> GNLPPEKKWLGTPIEEMRKMPRCGIHLPSLRPSASHTVTVRVDLLRAGEVPKPFPTHYKDLWDNKHVKMPCSEQNLYPVEDENGERTAGSRWELIQTALLNKFTRPQNLKDAILKYNVAYSKKWDFTALVDFWDKVLEEAEAQHLYQSILPDMVKIALCLPNICTQPIPLLKQKMNHSVTMSQEQIASLLANAFFCTFPRRNAKMKSEYSSYPDINFNRLFEGRSSRKPEKLKTLFCYFRRVTEKKPTGLVTFTRQSLEDFPEWERCEKPLTRLHVTYEGTIEGNGRGMLQVDFANRFVGGGVTGAGLVQNEIRFLINPELIVSRLFTEVLDHNECLIITGTEQYSEYTGYAETYRWARSHEDGSEKDDWQRRCTEIVAIDALHFRRYLDQFVPEKVRRELNKAYCGFLRPGVPSENLSAVATGNWGCGAFGGDARLKALIQILAAAAAERDVVYFTFGDSELMRDIYSMHTFLTERKLDVGKVYKLLLRYYNEECRNCSTPGPDIKLYPFIYHAVESSAET

Reversal of PARylation is predominantly carried out by poly(ADP-ribose) glycohydrolase (PARG) in nucleus and cytosol, whereas ADP-ribosylhydrolase 3 (ARH3) may play a role in mitochondrial PAR degradation. PARG comprises an N-terminal regulatory/targeting domain and a C-terminal catalytic domain. The mouse PARG catalytic domain has a bean-shaped structure, with the active site in a deep cleft in the middle on the abdominal side.

To understand what caused the activity difference between the mPARG E748N/Q and E749N/Q mutants, we solved the crystal structures of these mPARG mutants. Interestingly, while E748N and E749N mutants were completely dead, both E748Q and E749Q mutants still retained residual PARG activities. In contrast, the signature loops in E748N and E749N mutants have significantly different conformation from the wild type PARG. In wild-type PARG structure, Cβ and Cγ of both E748 and E749 residues are semi-buried. Mutation to Asn, which has both Cγ and Nγ linked to Cβ causes a spatial collision. Therefore, the conformation changes in this catalytic loop completely abolish activity of mPARG E748N and E749N mutants. To study the enzymatic mechanism of mPARG, we tried to soak the catalytic residue Glu748, Glu749 mutants E748N, E748Q, E749N and E749Q with the iso-ADPr, which may be the smallest PARG substrate containing the α(1→2) ribose-ribose glycosidic bond to be cleaved by PARG. In all above four PARG mutant crystal structures, we were not able to observe the electron density for iso-ADPr at the “active” site of mPARG. For E748N and E749N mutants, this may result from the conformational change in the active site associated with the mutation. Our work revealed precisely how some of the PARG mutations (e.g. E748N, E749N) disrupt the PARG activity through significant conformational changes in the PARG active site.>[2x]MDYKDDDDKAAAGSMIGGGIGISFRNEFFNPQTPVNIPVQGFSNGARLRLVLLPTSADSRFHINLRTPDDIVLHFNA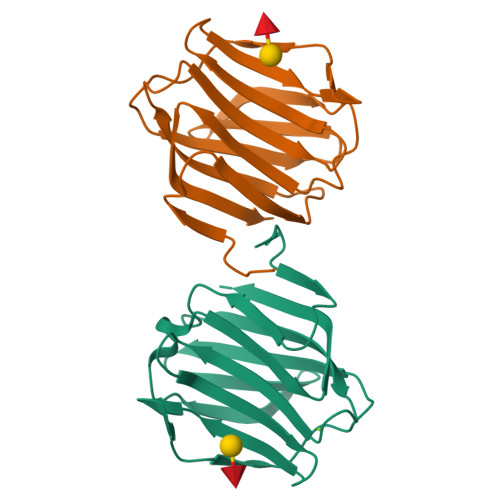RFDEGAVVNNSTSGGGWQSEDRHANPFQQNKIYTLEFVSNGGIISIFVNGAHFADFVERTPSHGVHLIEIEGGVHVHSAHVSH> MNITKPFPLPTGYFGIPLGLAALSLAWFHLENLFPAARMVSDVLGIVASAVWILFILMYAYKLRYYFEEVRAEYHSPVRFSFIALIPITTMLVGDILYRWNPLIAEVLIWIGTIGQLLFSTLRVSELWQGGVFEQKSTHPSFYLPAVAANFTSASSLALLGYHDLGYLFFGAGMIAWIIFEPVLLQHLRISSLEPQFRATMGIVLAPAFVCVSAYLSINHGEVDTLAKILWGYGFLQLFFLLRLFPWIVEKGLNIGLWAFSFGLASMANSATAFYHGNVLQGVSIFAFVFSNVMIGLLVLMTIYKLTKGQFFLK

The helium path was used for collection of anomalous diffraction data at 5 keV for two proteins: thaumatin and the membrane protein TehA. Although anomalous signals from each individual crystal are very weak, robust anomalous signals are obtained from data assembled from micrometre-sized crystals. The thaumatin structure was determined from 15 microcrystals and the TehA structure from 18 microcrystals. These results demonstrate the usefulness of a helium environment in support of native-SAD phasing at 5 keV.

TehA is an uncharacterized candidate for an ion channel as it is a bacterial homolog of the plant nitrate/chloride channel SLAC1. TehA consists of 314 residues, including 1 cysteine and 10 me­thio­nines. The calculated Bijvoet difference ratio is 1.8% at 5 keV. To remove statistically incompatible crystals, we performed crystal rejection. After rejection of 5 crystals out of 23, the 18-crystal dataset showed excellent CC1/2 and R split values, indicating high data quality [Figs. 4(a) and 4(b)]. BUCCANEER was able to build 300 out of 314 residues automatically. The refined structure has an R/R free of 0.17/0.22, indicating high map quality [Fig. 5(c)]. The f″ values of peaks 9 and 10 were very close to the calculated f″ values of Cl− and Zn2+ at 5 keV. The anomalous peaks 9 and 10 are coordinated by a nearby nitro­gen atom of the main chain or a Lys residue within a 3.2 Å distance [Figs. 7(a) and 7(b)], revealing that the two peaks should come from Cl− but not Zn2+. Interestingly, Na+ is located on the threefold axis of the TehA trimer, suggesting that Na+ may possibly be involved in TehA function.> GSGPTYCWNEANNPGGPNRCSNNKQCDGARTCSSSGFCQGT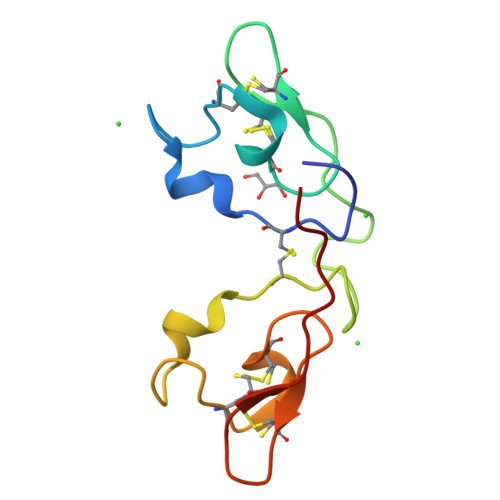SRKPDPGPKGPTYCWDEAKNPGGPNRCSNSKQCDGARTCSSSGFCQGTAGHAAA>[2x]GAMALPSGSDPAFSQPKSVLDAGLTCQGASPSSVSKPILLVPGTGTTGPQSFDSNWIPLSAQLGYTPCWISPPPFMLNDTQVNTEYMVNAITTLYAGSGNNKLPVLTVCQGGLVAQWGLTFFPSIRSKVDRLMAFAPDYKGTVLAGPLDALAGSAPSVWQQTTGSALTTALRNAGGLTQIVPTTNLYSATDEIVQPQVSNSPLDSSYLFNGKNVQAQAVCGPLFVIDHAGSLTSQFSYVVGRSALRSTTGQARSADYGITDCNPLPANDLTPEQKVAAAALLAPYYAAIVAGPKQNCEPDLMPYARPFAVGKRTCSGIVTP

Here, we choose lipase B from Candida antarctica (CALB), as the model enzyme, in which Asp187-His224-Ser105 is the catalytically active triad. Lipases function according to the classical Ser-His-Asp catalytic triad mechanism. In the present study we propose that the Ser → Cys conversion in lipases may lead to high activity by accurate manipulation of the local environment surrounding the hybrid Cys-His-Asp triad, enabled by laboratory evolution. We succeed in evolving cysteine-CALB mutants that are even more active than WT CALB.

In order to gain insight into the basis of increased activities of QW4 and QW10, the crystal structures of both enzymes were solved and refined to 1.85 and 1.88 Å resolution, respectively. Surprisingly, Cys105 in variant QW4 appeared to be oxidized to the respective sulfinic acid. Directed evolution of cysteine-CALB with generation of mutant QW4 led to a distinct improvement of activity for a range of bulky substrates, which are not well accepted by WT CALB. The raised mobility of loop 137–150 in QW4 and QW10 enables ready entry of bulky substrates, which can be attributed to the introduction of the V149G mutation. Interestingly, the nucleophile exchange (S105C) in QW4 results in a conformational change of helix 277–288, compared with QW10 or WT. While the helixes of QW10 and WT CALB are well superimposable, the helix section P280-Y282 of QW4 is deformed and shifted toward the active site, with an additional H-bond between Y281 and E188 formed. This conformational change also induces loop 289–294 next to helix 277–288 to shift by about 3.8 Å towards the solvent.> MRGSHHHH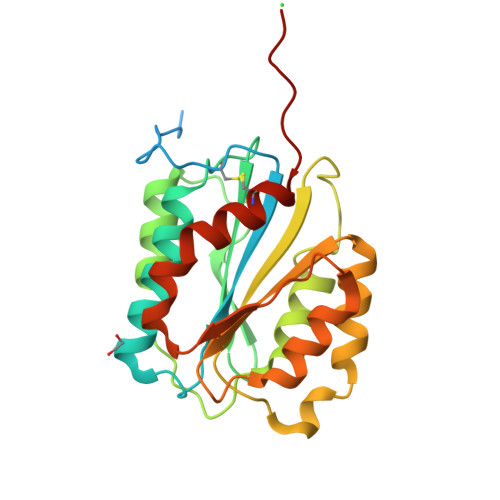HHGSQEPGGLVVPPTDAPVSPTTLYVEDISEPPLHDFYCSRLLDLVFLLDGSSRLSEAEFEVLKAFVVDMMERLRISQKWVRVAVVEYHDSSHAYIGLKDRKRPSELRRIASQVKYAGSQVASTSEVLKYTLFQIFSKIDRPEASRIALLLMASQEPQRMSRNFVRYVQGLKKKKVIVIPVGIGPHANLKQIRLIEKQAPENKAFVLSSVDELEQQRDEIVSYLCDLAPEAPPPTLPPKLN> MSEKTTKGVQLLRGDPKKAIVRLSIPMMIGMSVQTLYNLADGIWVSGLGPESLAAVGLFFPVFMGIIALAAGLGVGTSSAIARRIGARDKEGADNVAVHSLILSLILGVTITITMLPAIDSLFRSMGAKGEAVELAIEYARVLLAGAFIIVFNNVGNGILRGEGDANRAMLAMVLGSGLNIVLDPIFIYTLGFGVVGAAYATLLSMVVTSLFIAYWLFVKRDTYVDITLRDFSPSREILKDILRVGLPSSLSQLSMSIAMFFLNSVAITA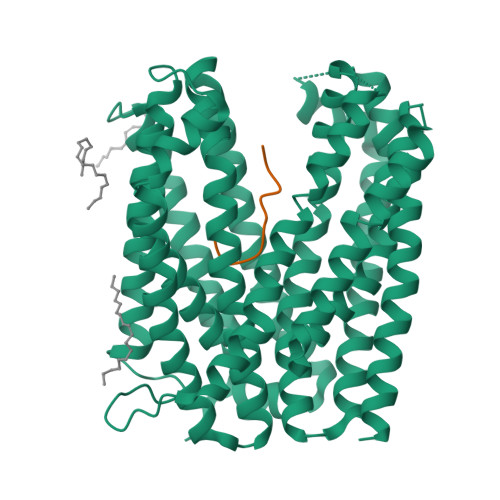GGENGVAVFTSAWRITMLGIVPILGMAAATTSVTGAAYGERNVEKLETAYLYAIKIAFMIELAVVAFIMLFAPQVAYLFTYSESAQVIKGDLISALRTLPVFLVLTPFGMMTSAMFQGIGEGEKSLILTIFRTLVMQVGFAYIFVHYTTLGLRGVWIGIVIGNMVAAIVGFLWGRMRISALKKTSATGGKR;> XFVYSAVCAAAA>[2x]MGSSHHHHHHSQDPMTDSTTHYTRPDVAAFLAFLNAQEGPKMEEMPPA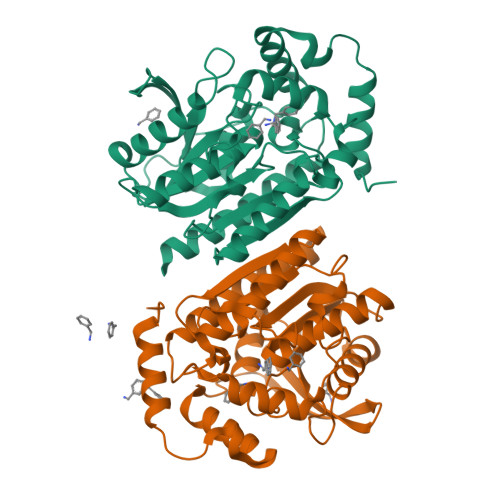GAREMMRVMGQLADVPRGEIAKVEDRMIPGPDGDIPIRLYDNRPDREAGPVMVFYHGGGWVIGDLETHDPYCAEAARILDMPVIAIDYRLAPEHPFPAAPIDCEAATRWVADNIACTGLVLSGDSAGGNLTIVTALALRDEPAAKPVIAIHPIYPAVTTHNDWQSYRDFGEGHLLTEGSMTWFGNHYAADPADRRAAPIDFPADGLPPTLLITASLDPLRDQGRAYAAKLIEAGVPTTYREAKGTIHGYICLAQGIPSAKDDIRGALTVLKAIVAEATGAA>ACKYDFATSVLFTEAELHTRMRGVAQRIADDYSNCNLKP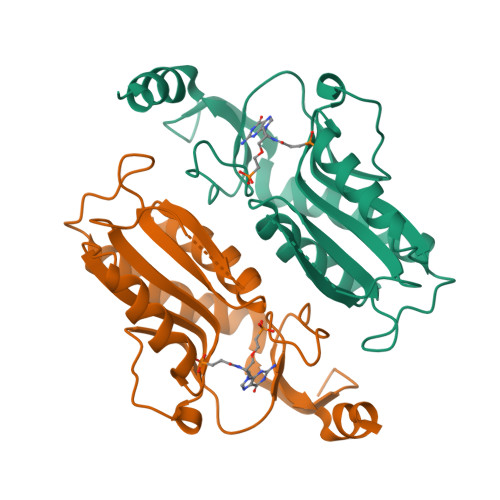LENPLVIVSVLKGSFVFTADMVRILGDFGVPTRVEFLRASSYGHDTKSCGRVDVKADGLCDIRGKHVLVLEDILDTALTLREVVDSLKKSEPASIKTLVAIDKPGGRKIPFTAEYVVADVPNVFVVGYGLDYDQSYREVRDVVILKPSVYETWGKELERRKA[4x]UspC from Mtb is a 441-amino acid protein that has been previously identified in bioinformatics analyses as a putative active importer of carbohydrates across the inner-membrane of the Mtb cell wall. The uspC gene forms part of a putative three-gene operon, uspABC, of which uspA and uspB encode the membrane-spanning subunits of the transporter, while uspC is a homologue of ABC transporter-linked solute-binding proteins. The fold of UspCNt follows the architecture of periplasmic binding proteins for bacterial ABC transporters, consisting of two subdomains or lobes that enclose the putative carbohydrate-binding cleft in the centre of the molecule. In conclusion, our data strongly indicate that Mtb-UspC is a carbohydrate-binding unit of the essential UspABC transporter system, with a substrate preference for sugars containing an amino group at the C2 or C3 position.

UspCNt readily formed crystals in vapour diffusion experiments using a commercial sparse matrix screen. Phases were determined by single-wavelength anomalous diffraction data to 2.6 Å, exploiting the anomalous signal from bound iodine ions. The structural model was refined against a native dataset (apo tetragonal) to a resolution of 1.5 Å. The UspCNt structure determined represents the ligand-free form and the model comprises residues 34–441, plus six additional residues of the partially ordered C-terminal affinity tag. UspCNt crystallized in two different crystal lattices. The tetragonal crystal form (space group P41) contained one copy of UspCNt in the crystallographic asymmetric unit (ASU), whereas the monoclinic crystal form (space group P21) contained two copies. The subdomains are joined by a central flexible hinge-linker that is localized around residues Asp145, Thr321 and Gly379. The molecular surface of UspCNt shows a prominent cleft between the two subdomains, which is characteristic for periplasmic substrate binding proteins of ABC transporters. The cleft is lined by several aromatic side chains, which affords the potential to form π-stacking interactions with carbohydrate moieties.

> PRGGKIVVTVRLWDEPIAAAYRQSFAAFTRSHPDIEVRTNLVAYSTYFETLRTDVAGGSADDIFWLSNAYFAAYADSGRLMKIQTDAADWEPAVVDQFTRSGVLWGVPQLTDAGIAVFYNADLLAAAGVDPTQVDNLRWSRGDDDTLRPMLARLTVDADGRTANTPGFDARRVRQWGYNAANDPQAIYLNYIGSAGGVFQRDGKFAFDNPGAIEAFRYLVGLINDDHVAPPASDTNDNGDFSRNQFLAGKMALFQSGTYSLAPVARDALFHWGVAMLPAGPAGRVSVTNGIAAAGNSASKHPDAVRQVLAWMGSTEGNSYLGRHGAAIPAVLSAQPVYFDYWSARGVDVTPFFAVLNGPRIAAPGGAGFAAGQQALEPYFDEMFLGRGDVTTTLRQAQAAANAATQRKLAAALEHHHHHH> RQLTVLERVAPTITGNLENQTTSIGESIEVSCTASGNPPPQIM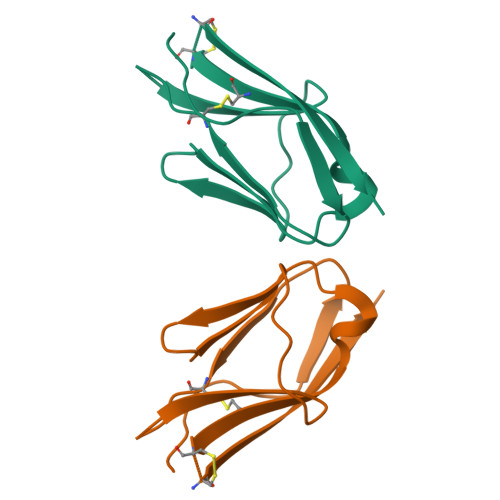WFKDNETLVEDSGIVLKDGNRNLTIRRVRKEDEGLYTCQACSVLGCAKVEAFFIIEGAQEKTNLE>KGGWFGKHRGQGGSNPKFENIAEGLRALLARSHVERTTDEGTWVAGVFVYGGSKTSLYNLRRGTALAIPQ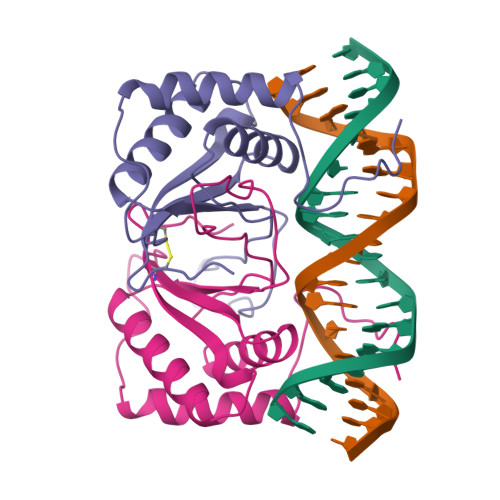CRLTPLSRLPFGMAPGPGPQPGPLRESIVCYFMVFLQTHIFAEVLKDAIKDLVMTKPAPTCNIRVTVCSFDDGVDLP[2x]> AMAKDSKAPVVEIFDERDGCTSAGSTGKASDAGEKGLLV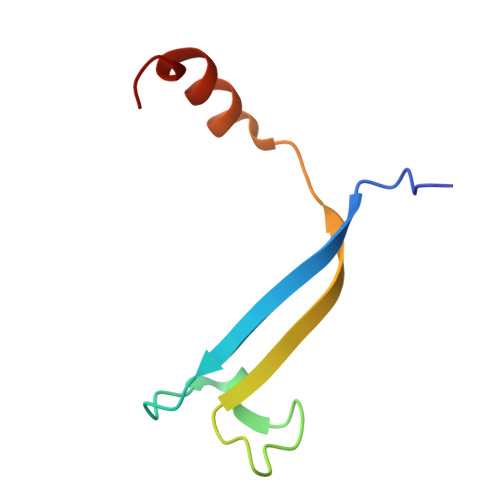KVSMQKVGYNAIMAKSVAASYMNA2-(6-AMINO-2-FLUORO-PURIN-9-YL)-5-HYDROXYMETHYL-TETRAHYDRO-FURAN-3,4-DIOL 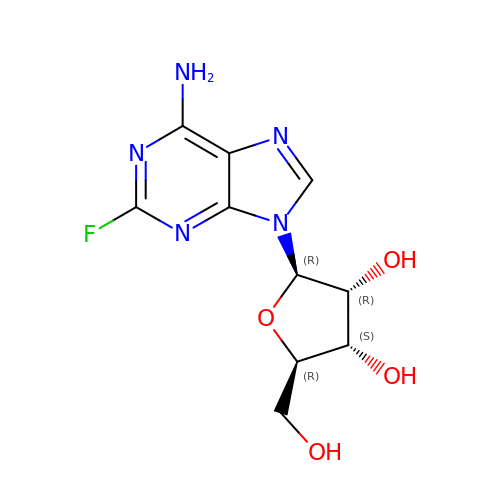| C10 H12 F N5 O4 | HBUBKKRHXORPQB-UUOKFMHZSA-N>[2x]GSHSLRYFFTWSTAGSGIPEFVAVGYVDDQQFVQYDSDRKEMIPRQRWVKESEGPEYWERETQTLRGWEPWGKANIDILSKRTNQTGGIHTYQLMCGCELRDDGSSNTGFVQHAWDSTDFISLDKDKMVWVTPVTWGEITKNKWDRDMAFNQGTKGYLEGICIEWLQKYLKNGNVELRPVKPSVTFTSVRGNKQLSCVATGFYPHSIEVNLFRDSAKIDETESTGVRPNHDGSYQIHR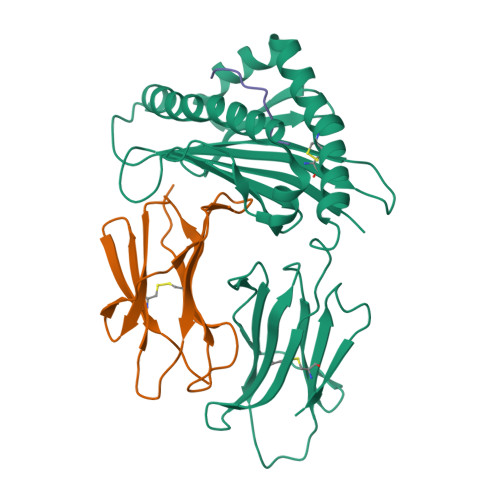STEFDPNSQAKYSCVVDHDGLGQQLVVFY;>[2x]ATSSPNVQVYTYKLIKEGESNVLLCHAKDFSPPNIKLELLENGRIIPNTTQSDLSFESDWSFKLTRYVEFTPQSGYKYSCMVTHNGDSKEIQLDRY;>[2x]FANFFIRGL> ADLALGAQVFNGNCAACHMGGRNSVMPEKTLDKAALEQYL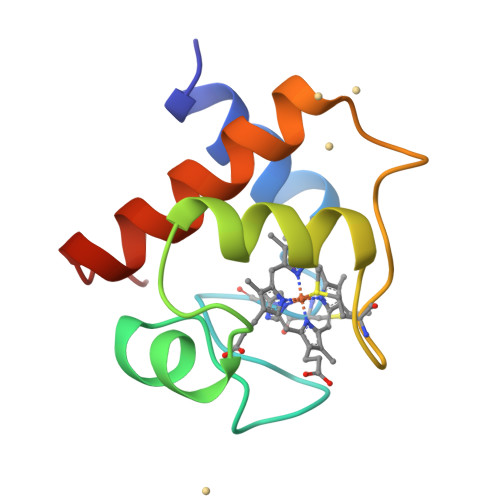DGGFKVESIIYQVENGKGAMPAWADRLSEEEIQAVAEYVFKQATDAAWKY> MGKDQLDFSHFDKAFENKYDIVAPEFGDLHQKRAEFIAKNQGTYRPVPLVPNNIKGLIPKTCRLPATRNWYRRTSSFERNGFFNIHTPVLNTKMIPWLLFIVL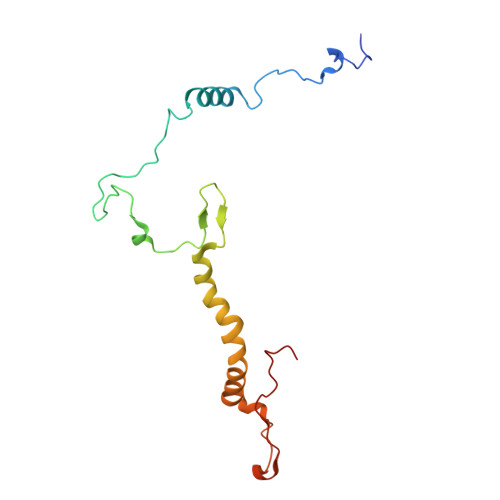TWGWSSFQIGGYNYERFDDNGERRNTLYWKLSPVEFPQSKLWNRPS>MRITFNDVKTSLGITESYDIVNAIRNSQGDNFKSYVPLATANNVAEVGAGILINQTVQNDFITSLVDRIGLVVIRQVSLNNPLKKFKKGQIPLGRTIEEIYTDITKEKQYDAEEAEQKVFEREMPNVKTLFHERNRQGFYHQTIQDDSLKTAFVSWGNFESFVSSIINAIYNSAEVDEYEYMKLLVDNYYSKGLFTTVKIDEPTSSTGALTEFVKKMRATARKLTLPQGSRDWNSMAVRTRSYMEDLHLIIDADLEAELDVDVLAKAFNMNRTDFLGNVTVIDGFASTGLEAVLVDKDWFMVYDNLHKMETVRNPRGLYWNYYYHVWQTLSVSRFANAVAFVSGDVPAVTQVIVSPNIAAVKQGGQQQFTAYVRATNAKDHKVVWSVEGGSTGTAITGDGLLSVSGNEDNQLTVKATVDIGTEDKPKLVVGEAVVSIRPNNASGGAQA[235x];>MMVSFTARAKSNVMAYRLLAYSQGDDIIEISHAAENTIPDYVAVKDVDKGDLTQVNMYPLAAWQVIAGSDIKVGDNLTTGKDGTAVPTDDPSTVFGYAVEEAQEGQLVTLVISRSKEISIEVEDIKDAGDTGKRLLKINTPSGARNIIIENEDAKALINGETTNTNKKNLQDLLFSDGNVKAFLQATTTDENKTALQQLLVSNADVLGLLSGNPTSDNKINLRTMIGAGVPYSLPAATTTTLGGVKKGAAVTASTATDVATAVKDLNSLITVLKNAGIISL[165x]

The bacteriophage ϕ29, a representative of bacteriophages with a short non-contractile tail, has an ~19 kb dsDNA genome encoding ~20 proteins. Both 5ʹ ends of the genome are covalently connected to the terminal protein gene product 3 (gp3). ϕ29 infects the Gram-positive Bacillus subtilis cells by injecting the genome–gp3 complex into the host-cell cytoplasm using a short non-contractile tail, leaving the genome emptied virion on the cell surface. Here, we report the cryo-electron microscopy (cryo-EM) structural studies of the ϕ29 prohead, the mature and the genome-emptied virions at near-atomic resolutions up to 3.2 Å. Our results show structural details of the complex capsid, the DNA packaging motor and the entire tail machinery, and provide a molecular basis for understanding the assembly, maturation and infection mechanisms of the bacteriophage ϕ29.

We calculated the cryo-electron microscopy (cryoEM) reconstructions of the ϕ29 prohead, the mature head and the genome emptied head to a resolution of 3.6, 3.2, and 3.2 Å, respectively. The complete mature and the genome-emptied virion models each consist of 235 copies of the major capsid protein gp8, 165 copies of the minor capsid protein gp8.5, 12 copies each of the connector protein gp10 and the tail protein gp11, 36 copies of the tail appendage protein gp12* and 6 copies of the tail knob protein gp9. Structural comparisons of the heads showed overall small differences between the heads (an average r.m.s.d of 0.7 Å). Structural comparisons of the mature and the genome-emptied heads showed that the equatorial part of the genome-emptied head expanded slightly after the ejection of the genome. However, the icosahedral end caps shrink upon the release of the inner pressure, showing the elasticity of the capsid. The ϕ29 capsid undergoes only miniscule conformational changes upon genome loading and release and does not generate sufficiently large holes for the exit of the scaffolding protein.> GSMYLINQNGWIEVICGSMFSGKSEELIRRVRRTQFAKQHAIVFKPCIDNRYSEEDVVSHNGLKVKAVPVSASKDIFEHITEELDVIAIDEVQFFDGDIVEVVQVLANRGYRVIVAGLDQDFRGLPFGQVPQLMAIAEHVTKLQAVCSVCGSPASRTQRLIDGEPAAFDDPIILVGASESYEPR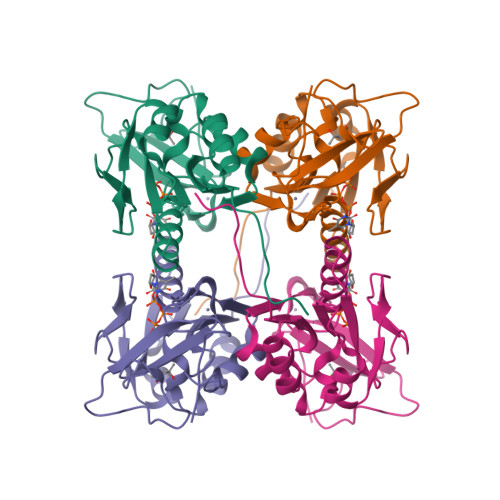CRHCHAVPANKDK> NYRSRAAYKLIELDNKYLFLKKNKIILDIGCYPGSWCQVILERTKNYKNKIIGIDKKIMDPIPNVYFIQGEIGKDNMNNIKNINYID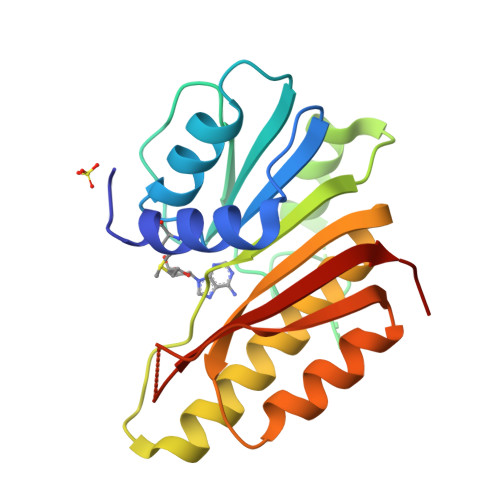NMNNNSVDYKLKEILQDKKIDIILSDAAVPCIGNKIDDHLNSCELTLSITHFMEQYINIGGTYIVKMYLGSQTNNLKTYLKGMFQLVHTTKPKASRNESREIYLVCKNFLGRKK>[8x]MN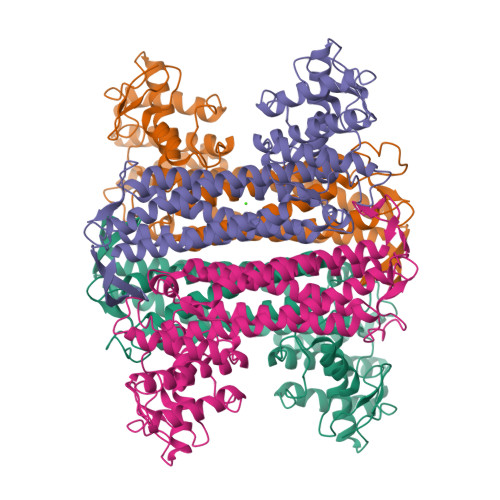TDVRIEKDFLGEKEIPKDAYYGVQTIRATENFPITGYRIHPELIKSLGIVKKSAALANMEVGLLDKEVGQYIVKAADEVIEGKWNDQFIVDPIQGGAGTSINMNANEVIANRALELMGEEKGNYSKISPNSHVNMSQSTNDAFPTATHIAVLSLLNQLIETTKYMQQEFMKKADEFAGVIKMGRTHLQDAVPILLGQEFEAYARVIARDIERIANTRNNLYDINMGATAVGTGLNADPEYISIVTEHLAKFSGHPLRSAQHLVDATQNTDCYTEVSSALKVCMINMSKIANDLRLMASGPRAGLSEIVLPARQPGSSIMPGKVNPVMPEVMNQVAFQVFGNDLTITSASEAGQFELNVMEPVLFFNLIQSISIMTNVFKSFTENCLKGIKANEERMKEY>[2x]GPGTNRSLIVTTLLEEPFVMFRKSDRTLYGNDRFEGYCIDLLKELAHILGFSYEIRLVEDGKYGAQDDKGQWNGMVKE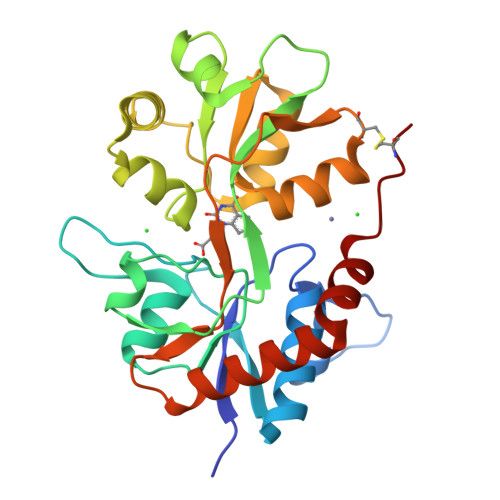LIDHKADLAVAPLTITHVREKAIDFSKPFMTLGVSILYRKGTPIDSADDLAKQTKIEYGAVKDGATMTFFKKSKISTFEKMWAFMSSKPSALVKNNEEGIQRTLTADYALLMESTTIEYITQRNCNLTQIGGLIDSKGYGIGTPMGSPYRDKITIAILQLQEEDKLHIMKEKWWRGSGCP>[2x]MAITIDSARRIFPNTLQADAVPALTARFNQLSAEDQLAWTWFAFLEMGKTITVAAPGAASMQF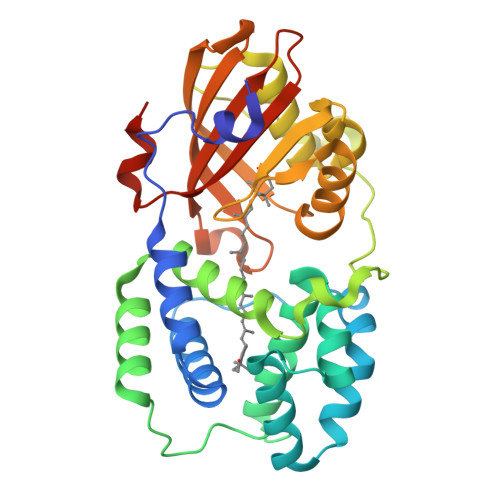AEGILKQIKEMTFEEQTQVMCDLANHTDTPICRTYATWSPNIKLGFWNQLGEWMEQGAVAPIPAGYQLSANANAVLETLKSLDQGQQITVLRSSVVDMGFDAAKLDGYTRVAEPLVAPKDISQRVQVTIEGINNSTVLNYMNNLNANDFDELIKLFVEDGALQPPFQRPIVGKDAILRFFREECQNLNLLPERGVAEPADDGYTQVKVTGKVQTPWFGAAVGMNMAWRFLLNPQGKIFFVAIDLLASPKELLNLVRHHHHHH>ASYGKKTQMSILEQRESLPIYKLKEQLVQAVHDNQILIVIGETGSGKTTQITQYLAEAGYTSRGKIGCTQPRRVAAMSVAKRVSEEFGCCLGQEVGYTIRFEDCTSPETVIKYMTDGMLLRECLIDPDLTQYAIIMLDEAHERTIHTDVLFGLLKKTVQKRQDMKLIVTSATLDAVKFSQYFYEAPIFTIPGRTYPVEILYTKEPETDYLDASLITVMQIHLTEPPGDILVFLTGQEEIDTACEILYERMKSLGPDVPELIILPVYSALPSEMQTRIFDPAPPGSRKVVIATNIAETSLTIDGIYYVVDPGFVKQKVYNSKTGIDQLVVTPISQAQAKQRAGRAGRTGPGKCYRLYTERAYRDEMLTTNVPEIQRTNLASTVLSLKAMGINDLLSFDFMDAPPMETLITAMEQLYTLGALDDEGLLTRLGRRMAEFPLEPMLCKMLIMSVHLGCSEEMLTIVSMLSVQNVFYRPKDKQALADQKKAKFHQTEGDHLTLLAVYNSWKNNKFSNPWCYENFIQARSLRRAQDIRKQMLGIMDRHKLDVVSCGKSTVRV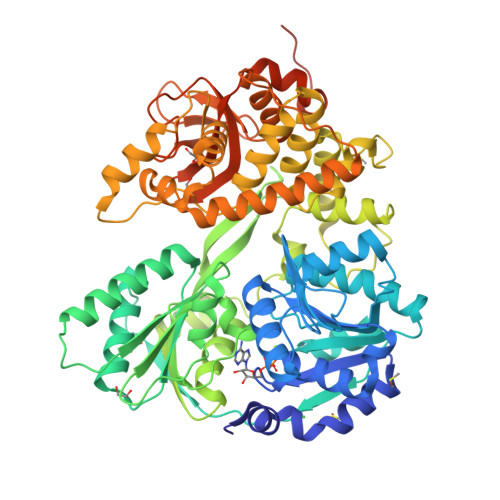QKAICSGFFRNAAKKDPQEGYRTLIDQQVVYIHPSSALFNRQPEWVVYHELVLTTKEYMREVTTIDPRWLVEFAPAFFKVSDPTKLSKQKKQQRLEPLYNRYEEPNAWRISRAFRRR[4x]>[2x]MRERPHT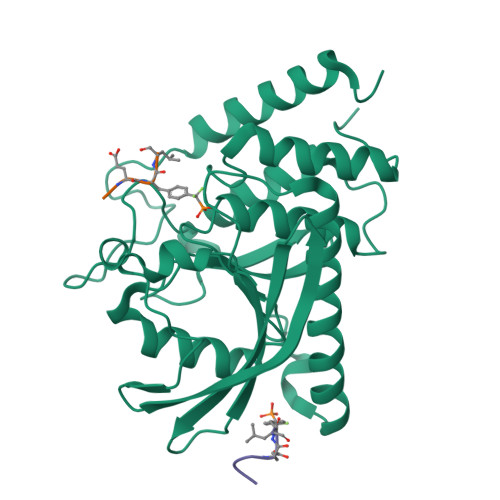SGHHGAGEARATAPSTVSPYGPEARAELSSRLTTLRNTLAPATNDPRYLQACGGEKLNRFRDIQCRRQTAVRADLNANYIQVGNTRTIACQYPLQSQLESHFRMLAENRTPVLAVLASSSEIANQRFGMPDYFRQSGTYGSITVESKMTQQVGLGDGIMADMYTLTIREAGQKTISVPVVHVGNWPDQTAVSSEVTKALASLVDQTAETKRNMYESKGSSAVADDSKLRPVIHCRAGVGRTAQLIGAMCMNDSRNSQLSVEDMVSQMRVQRNGIMVQKDEQLDVLIKLAEGQGRPLLNS;>DADEYLX[4x]>MAQGTLYIVSAPSGAGKSSLIQALLKTQPLYDTQVSVSHTTRQPRPGEVHGEHYFFVNHDEFKEMISRDAFLEHAEVFGNYYGTSREAIEQVLATGVD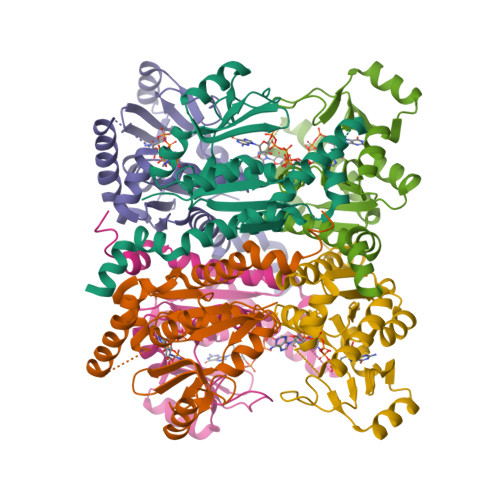VFLDIDWQGAQQIRQKMPHARSIFILPPSKIELDRRLRGRGQDSEEVIAKRMAQAVAEMSHYAEYDYLIVNDDFDTALTDLKTIIRAERLRMSRQKQRHDALISKLLAD[2x]The guanidine-II (mini-ykkC) riboswitch is the smallest of the guanidine-responsive riboswitches, comprising two stem loops of similar sequence. The guanidine riboswitches bind the guanidinium cation such that the level of expression of genes that deal with guanidine toxicity is upregulated. Crystal structures of these stem loops show that they are intrinsically disposed to dimerization by loop-loop interaction. The loop-loop interaction creates binding sites for two guanidine molecules, and thus the folded conformation of the RNA is stabilized by guanidine binding, which leads to the increased level of gene expression.

In addition, we have solved the structure of a guanidine-II riboswitch P1 8-bp stem loop from Escherichia coli bound to guanidine. The structure is closely similar to that of the G. violaceus RNA, with an RMSD of 0.28 Å.

>[4x]UUUGCAGGACGACCUGCAAA1-[3-(trifluoromethyl)phenyl]-1H-pyrazol-4-ol 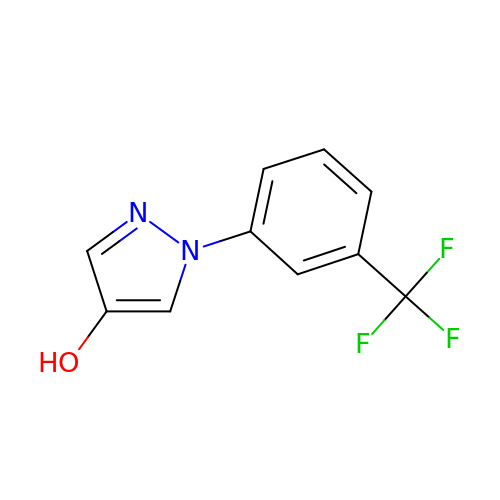| C10 H7 F3 N2 O | SGZRMGCFXYGLQZ-UHFFFAOYSA-N> MAVPIQKVQDDTKTLIKTIVTRINDISHTQS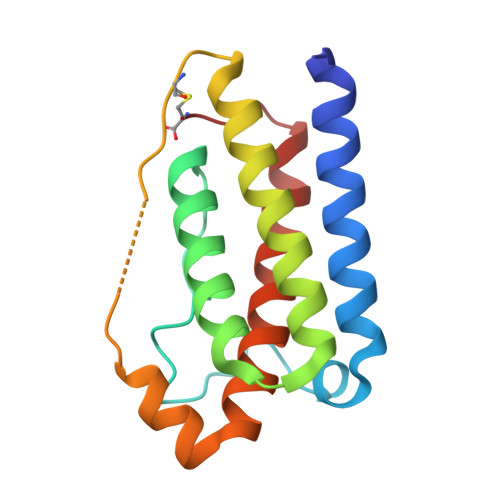VSAKQRVTGLDFIPGLHPILSLSKMDQTLAVYQQVLTSLPSQNVLQIANDLENLRDLLHLLAFSKSCSLPQTSGLQKPESLDGVLEASLYSTEVVALSRLQGSLQDILQQLDVSPEC4-[4-[5-[imidazo[1,2-a]pyridin-6-ylmethyl(methyl)amino]-1,3,4-oxadiazol-2-yl]-3-methyl-phenyl]-2,5-dimethyl-pyrazole-3-carbonitrile 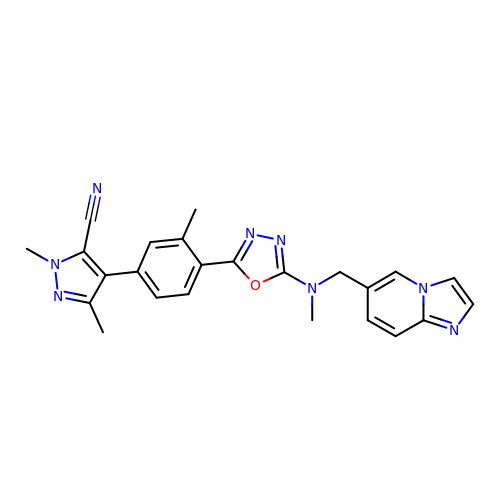| C24 H22 N8 O | LOJVVUQLHLHRMD-UHFFFAOYSA-N> GSGPAFESY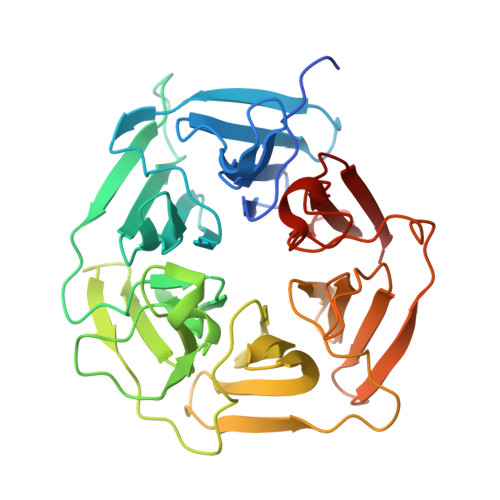ESMELACPAERSGHVAVSDGRHMFVWGGYKSNQVRGLYDFYLPREELWIYNMETGRWKKINTEGDVPPSMSGSCAVCVDRVLYLFGGHHSRGNTNKFYMLDSRSTDRVLQWERIDCQGIPPSSKDKLGVWVYKNKLIFFGGYGYLPEDKVLGTFEFDETSFWNSSHPRGWNDHVHILDTETFTWSQPITTGKAPSPRAAHACATVGNRGFVFGGRYRDARMNDLHYLNLDTWEWNELIPQGICPVGRSWHSLTPVSSDHLFLFGGFTTDKQPLSDAWTYCISKNEWIQFNHPYTEKPRLWHTACASDEGEVIVFGGCANNLLVHHRAAHSNEILIFSVQP> MTTQLRYENNDDDERVEYNLFTNRSTMMANFEEWIKMATDNKINSRNSWNFALIDYFYDLDVLKDGENNINFQKASATLDGCIKIYSSRVDSVTTETGKLLSGLAQRKTNGASNGDDSNGGNGEGLGGDSDEANIEIDPLTGMPISNDPDVNNTRRRVYNRVLETTLVEFETIKMKELDQELIIDPLFKKALVDFD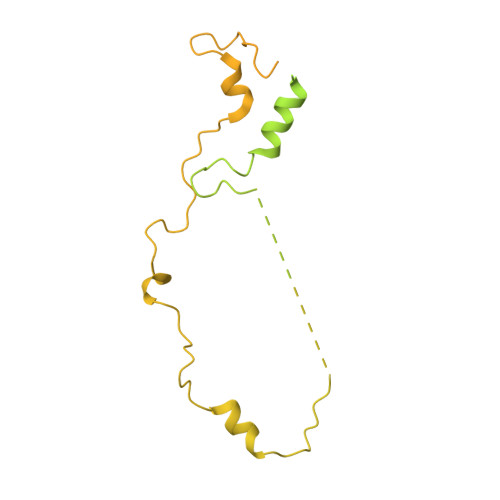EGGAKSLLLNTLNIDNTARVIFDASIKDTQNVGQGKLQRKEEELIERDSLVDDENEPSQSLISTRNDSTVNDSVISAPSMEDEILSLGMDFIKFDQIAVCEISGSIEQLRNVVEDINQAKDFIENVNNRFDNFLTEEELQAAVPDNAEDDSDGFDMGMQQELCYPDENHDNTSHDEQDDDNVNSTTGSIFEKDLMAYFDENLNRNWRGREHWKVRNFKKANLVNKESDLLEETRTTIGDTTDKNTTDDKSMDTKKKHKQKKVLEIDFFKTDDSFEDKVFASKGRTKIDMPIKNRKNDTHYLLPDDFHFSTDRITRLFIKPGQKMSLFSHRKHTRGDVSSGLFEKSTVSANHSNNDIPTIADEHFWADNYERKEQEEKEKEQSKEVGDVVGGALDNPFEDDMDGVDFNQAFEGTDDNEEASVKLDLQDDEDHKFPIRENKVTYSRVSKKVDVRRLKKNVWRSINNLIQEHDSRKNREQSSNDSETHTEDESTKELKFSDIIQGISKMYSDDTLKDISTSFCFICLLHLANEHGLQITHTENYNDLIVNYEDLATTQAAS>SMDKLKKIDQTIHAFYCEKAVISEKLNEAVLYSINAGGKRIRPILFLEVIEALQIPLTESHFKAAAALEMIHTGSLIHDDLPAMDNDDYRRGQLTNHKKFDEATAILAGDSLFLDAFGMLAETDFPTDVTVDLVRSLSSASGTFGMVGGQMLDMA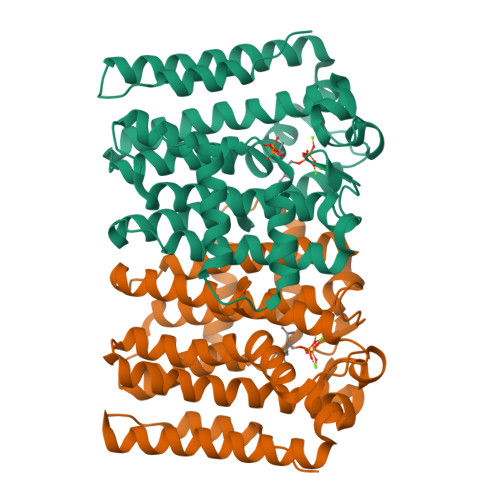AEGKKLNLKNLQLIHRHKTGQLLAYPFWAAARVAQLDENLLATFLEIGMIIGLAFQVRDDILDITANFEEIGKTPKKDVMAEKMTYPHLLGLNESYQILDESLDQAEAILRKLSDEIAFAPQKILSLIERLRLDA[2x]> SNANYMETGDQRFGDLVFRQLAPNVWQHTSYLDMPGFGAVASNGLIVRDGGRVLVVDTAWTDDQTAQILNWIKQEINLPVALAVVTHAHQDKMGGMDALHAAGIAT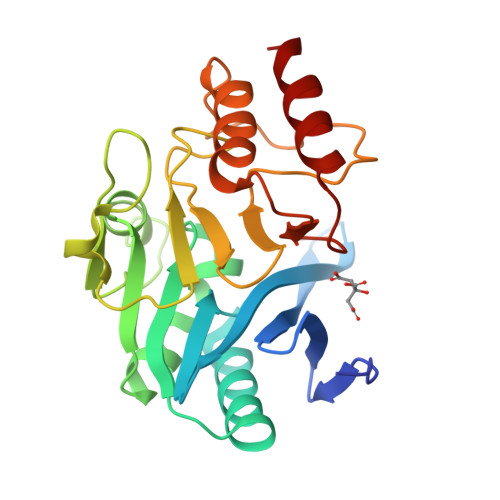YANALSNQLAPQEGMVAAQHSLTFAANGWVEPATAPNFGPLKVFYPGPGHTSDNITVGIDGTDIAFGGCLIKDSKAKSLGNLGDADTEHYAASARAFGAAFPKASMIVMSHSAPDSRAAITHTARMADKLR> GSHMTTPSHLSDRYELGEILGFGGMSEVHLARDLRDHRDVAVKVLRADLARDPSFYLRFRREAQNAAALNHPAIVAVYDTGEAETPAGPLPYIVMEYVDGVTLRDIVHTEGPMTPKRAIEVIADACQALNFSHQNGIIHRDVKPANIMISATNAVKVMDFGIARAIADSGNSVTQTAAVIGTAQYLSPEQARGDSVDARSDVYSLGCVLYEVLTGEPPFTGDSPDSVAYQHVREDPI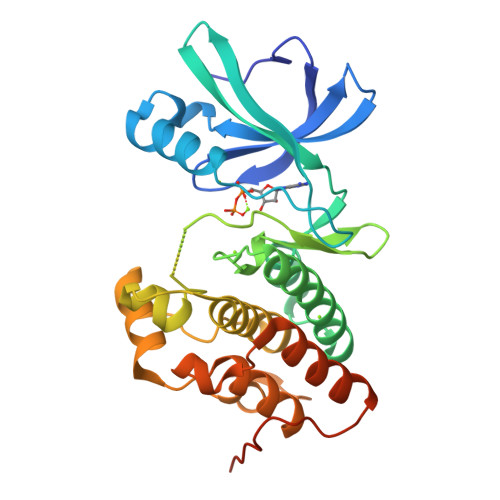PPSARHEGLSADLDAVVLKALAKNPENRYQTAAEMRADLVRVHNGEPPEAPKVLTDAERTSLLSSAAGNLSGPR>STPSIVIASAARTAVGSFNGAFANTPAHELGATVISAVLERAGVAAGEVNEVILGQVLPAGEGQNPARQAAMKAGVPQEATAWGMNQLAGSGLRAVALGMQQIATGDASIIVAGGMESMSMAPHCAHLRGGVKMGDFKMIDTMIKDGLTDAFYGYHMGTTAENVAKQWQLSRDEQDAFAVASQNKAEAAQKDGRFKDEIVPFIVKGRKGDITVDADEYIRHGATLDSMAKLRPAFDKEGTVTAGNASGLNDGAAA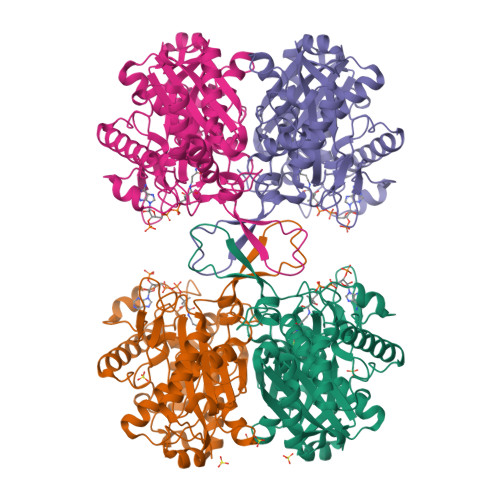ALLMSEAEASRRGIQPLGRIVSWATVGVDPKVMGTGPIPASRKALERAGWKIGDLDLVEANEAFAAQACAVNKDLGWDPSIVNVNGGAIAIGHPIGASGARILNTLLFEMKRRGARKGLATLCIGGGMGVAMCIESL[4x]> MLSSTALLLRGQYKTRLKKRMVGFIPKVIPRKIKNNMVALRSEANTGHMEGYLKTETERLDATGRKVQKVLWDPVLQRHCLFKETKIKGPFMTKSAI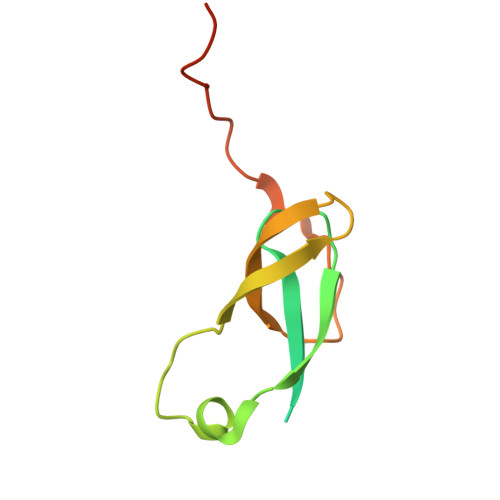AKKVDFPIGGAEKMLKK> AAPGKPTIAWGNTKFAIVEVDQAATAYNNLVKVKNAADVSVSWNLWNGDTGTTAKILLNGKEAWSGPSTGSSGTANFKVNKGGRYQMQVALCNADGCTASDATEIVVADTDGSHLAPLKEPLLEKNKPYKQNSGKVVGSYFVEWGVYGRNFTVDKIPAQNLTHLLYGFIPICGGNGINDSLKEIEGSFQALQRSCQGREDFKVSIHDPFAALQKAQKGVTAWDDPYKGNFGQLMALKQAHPDLKILPSIGGWTLSDPFFFMGDKVKRDRFVGSVKEFLQTWKFFDGVDIDWEFPGGKGANPNLGSPQDGETYVLLMKELRAMLDQLSAETGRKYELTSAISAGKDKIDKVAYNVAQNSMDHIFLMSYDFYGAFDLKNLGHQTALNAPAWKPDTAYTTVNGVNALLTQGVKPGKIVVGTAMYGRGWTGVNGYQNNIPFTGTATGPVKGTWENGIVDYRQIASQFMSGEWQYTYDATAEAPYVFKPSTGDLITFDDARSVQAKGKYVLDKQLGGLFSWEIDADNGDILN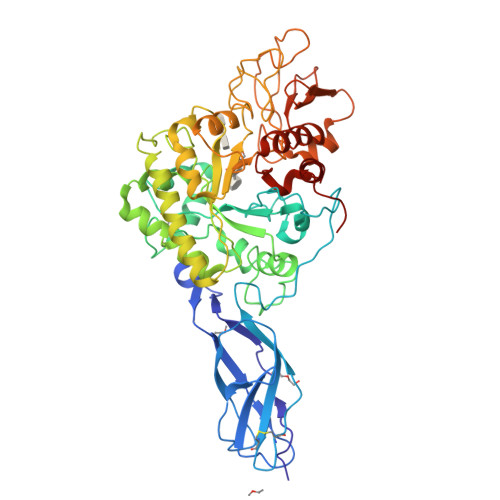SMNASLGNSAGVQ> GPVKTQEDLLPLVPEQVFVEMYEDMARRQTIEALVPAWDSDIIFKCLCYFHTLYPGLIPLETFPPATIFNFKQKIISILEDKKAVLRGEPIKGPLPICCSKENYRRHLQRTTLLPVFMWYHPTPKTLSDTMQTMKQLAIKGSVGASHWLLVIVDIQARRLVYFDSLYNYVMPPENMKKELQSFAQQLDQVYPAYDSKKFSVKIAAKEVIQRGSGSSCGAWCCQFLHWYLKDPLTDALNDLPVDSVERHENLASFVQACEAAVQDLPELSWPEA

CE clan proteases, specific hydrolases for ubiquitin-like modifications (SUMO and NEDD8) in eukaryotes, reportedly serve as bacterial effector proteins with deSUMOylase, deubiquitinase, or, even, acetyltransferase activities. Here, we characterize bacterial CE protease activities, revealing K63-linkage-specific deubiquitinases in human pathogens, such as Salmonella, Escherichia, and Shigella, as well as ubiquitin/ubiquitin-like cross-reactive enzymes in Chlamydia, Rickettsia, and Xanthomonas. Five crystal structures, including ubiquitin/ubiquitin-like complexes, explain substrate specificities and redefine relationships across the CE clan. A comparison to the previously determined SENP2-SUMO2 and NEDP1∼NEDD8 complexes (Reverter and Lima, 2004, Reverter et al., 2005, Shen et al., 2005) revealed differences among bacterial CE DUBs in three variable regions (VRs) near the substrate binding (S1) site that were arranged around a structurally conserved helix (constant region, CR).

We determined high-resolution crystal structures of the CE clan effectors SseL, RickCE, and ChlaDUB1. Interestingly, the remaining bacterial effectors SseL, ElaD, and ShiCE are Ub-specific proteases, and ChlaDUB1 and RickCE cleave both Ub- and, to a lesser extent, NEDD8-modified peptides. Like NEDP1, ChlaDUB1 can remove the C-terminal five amino acids from pro-NEDD8 with peptidase activity, but does not cleave the regulatory NEDD8 modification from the cullin RING ligase adaptor Cul1. A corresponding VR-1 region is absent in ChlaDUB1; interestingly, the ChlaDUB1 C terminus occupies this space instead. NEDP1 and ChlaDUB1 contain an insertion of 7 and 24 residues, respectively, in what is a short β-turn in the other structures. In contrast, ChlaDUB1 forms a helix that may serve a similar purpose in recognition of the Ub C terminus. Matching their specificity profiles, ChlaDUB1 and RickCE can both form covalent adducts with Ub and NEDD8 suicide probes. Deletion of the inserted VR-3 helix of ChlaDUB1 or the predicted VR-1 outside the crystallized boundaries of RickCE resulted in a total loss in recognition of the Ub/Ubl probes. The Ub/NEDD8 cross-reactive enzymes ChlaDUB1 and RickCE fall into their own clade.>MPVTINNFNYNDPIDNNNIIMMEPPFARGTGRYYKAFKITDRIWIIPERYTFGYKPEDFNKSSGIFNRDVCEYYDPDYLNTNDKKNIFLQTMIKLFNRIKSKPLGEKLLEMIINGIPYLGDRRVPLEEFNTNIASVTVNKLISNPGEVERKKGIFANLIIFGPGPVLNENETIDIGIQNHFASREGFGGIMQMKFCPEYVSVFNNVQENKGASIFNRRGYFSDPALILMHELIHVLHGLYGIKVDDLPIVPNEKKFFMQSTDAIQAEELYTFGGQDPSIITPSTDKSIYDKVLQNFRGIVDRLNKVLVCISDPNININIYKNKFKDKYKFVEDSEGKYSIDVESFDKLYKSLMFGFTETNIAENYKIKTRASYFSDSLPPVKIKNLLDNEIYTIEE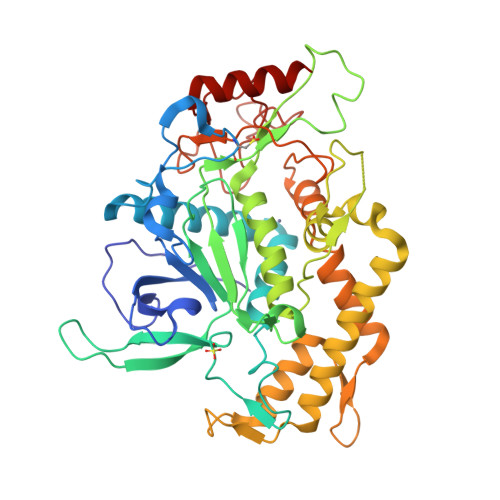GFNISDKDMEKEYRGQNKAINKQAYEEISKEHLAVYKIQMCKSVK[2x]Mammalian apurinic/apyrimidinic (AP) endonuclease 1 (APE1) is required for the repair of abasic sites and other DNA lesions and is an essential element of the base-excision repair (BER) and strand-break repair pathways. APE1 hydrolyzes the phosphodiester bond at abasic sites, producing 5′-deoxyribose phosphate (dRP) and the 3′-OH primer needed for repair synthesis, and is the major AP endonuclease in mammalian cells. APE1 also mediates the repair of single-strand and double-strand breaks by removing 3′-blocking groups (fragmented sugar moieties), again giving a 3′-OH for subsequent repair. APE1 possesses a remarkable degree of catalytic power and Mg2+ is an essential cofactor.

Here, we report the crystal structure of human APE1 solved at 1.92 Å resolution with a single Mg2+ ion bound in the active site. A construct of human APE1 that lacks the 38 N-terminal residues, APE1ΔN38, was crystallized under neutral pH conditions by sitting-drop vapor diffusion (at 22°C). The crystals belonged to the monoclinic space group C2, with three molecules per asymmetric unit. While some residues within the structured catalytic domain are absent in previously reported structures of DNA-free APE1, electron density is observed for all residues from Leu44 to the C-terminus (Leu318) in the structure reported here. The same octahedral metal-coordination geometry and ligands are observed in all three active sites of the asymmetric unit. The observation that DNA-free APE1 binds a single Mg2+ ion at the A site (Asp70 and Glu96) and that a second Mg2+ ion does not bind at the B site is consistent with the results of two previous NMR studies. One of the two residues that directly coordinate the Mg2+ ion, Glu96, is strictly conserved in the DNase I superfamily, while the other, Asp70, seems to be restricted to mammalian APE1. The carboxylate of Asp308 binds two of the four inner-sphere water molecules of Mg2+. The coordination mechanism for Mg2+ observed in the new structure differs substantially from that observed for Sm3+ and Pb2+ in previous structures of DNA-free APE1. Our structure (1.9 Å resolution) and previously determined structures of free APE1 (except for the two-Pb2+ structure) contain a water molecule at the ‘B’ site of the DNA-free enzyme and a second Mg2+ is not observed in the recently determined structure of the EP complex (2.4 Å resolution). Together, these observations argue against the idea that Mg2+ binds to both the A and B sites or that a single Mg2+ moves from the A site in the free enzyme to the B site in the ES complex to activate the water nucleophile and then back to the A site in the EP complex.

>[3x]GSHMASGEGPALYEDPPDQKTSPSGKPATLKICSWNVDGLRAWIKKKGLDWVKEEAPDILCLQETKCSENKLPAELQELPGLSHQYWSAPSDKEGYSGVGLLSRQCPLKVSYGIGDEEHDQEGRVIVAEFDSFVLVTAYVPNAGRGLVRLEYRQRWDEAFRKFLKGLASRKPLVLCGDLNVAHEEIDLRNPKGNKKNAGFTPQERQGFGELLQAVPLADSFRHLYPNTPYAYTFWTYMMNARSKNVGWRLDYFLLSHSLLPALCDSKIRSKALGSDHCPITLYLAL> PAQDNSRFVIRDRNWHPKALTPDYKTSIARSPRQALVSIPQSISETTGPNFSHLGFGAHDHDLLLNFNNGGLPIGERIIVAGRVVDQYGKPVPNTLVEMWQANAGGR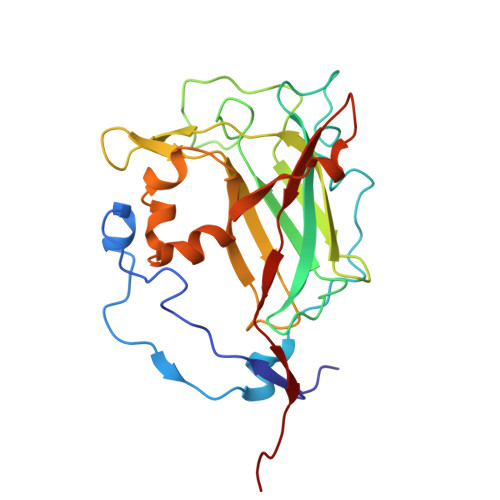YRHKNDRYLAPLDPNFGGVGRCLTDSDGYYSFRTIKPGPYPWRNGPNDWRPAHIHFGISGPSIATKLITQLYFEGDPLIPMCPIVKSIANPEAVQQLIAKLDMNNANPMDCLAYRFDIVLRGQRKTHFENC> SAMMYIQELRSGLRDMHLLSCLESLRVSLNNNPVSWVQTFGAEGLASLLDILKRLHDEKEETSGNYDSRNQHEIIRCLKAFMNNKFGIKTMLETEEGILLLVRAMDPAVPNMMIDAAKLLSALCILPQPEDMNE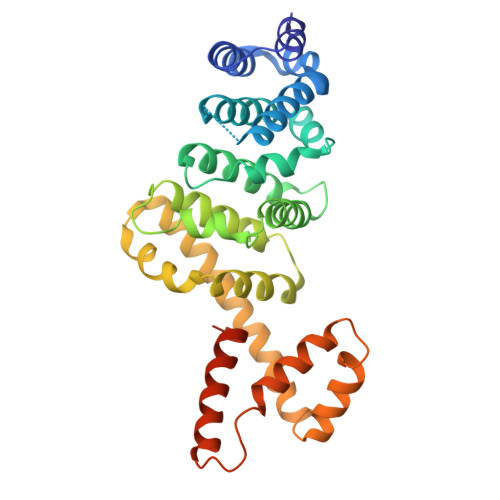RVLEAMTERAEMDEVERFQPLLDGLKSGTSIALKVGCLQLINALITPAEELDFRVHIRSELMRLGLHQVLQELREIENEDMKVQLCVFDEQGDEDFFDLKGRLDDIRMEMDDFGEVFQIILNTVKDSKAEPHFLSILQHLLLVRNDYEARPQYYKLIEECVSQIVLHKNGTDPDFKCRHLQID> GQRIRVR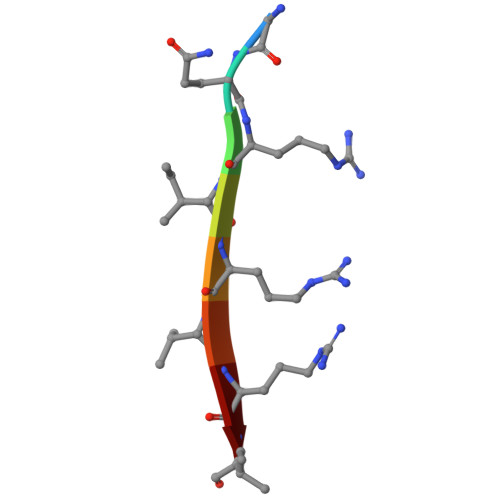I>GPLGSETITVPTPIKQIFSDDAFAETIKDNLKKKSVTDAVTQNELNSIDQIIANNSDIKSVQGIQYLPNVTKLFLNGNKLTDIKPLANLKNLGWLFLDENKVKDLSSLKDLKKLKSLSLEHNGISDINGLVHLPQLESLYLGNNKITDITVLSRLTKLDTLSLEDNQISDIVPLAGLTKLQNLYLSKNHISDLRALAGLKNLDVLELFSQECLNKPINHQSNLVVPNTVKNTDGSLVTPEIISDDGDYEKPNVKWHLPEFTNEVSFIFYQPVTIGKAKARFHGRVTQPLKEVYTVSYDVDGT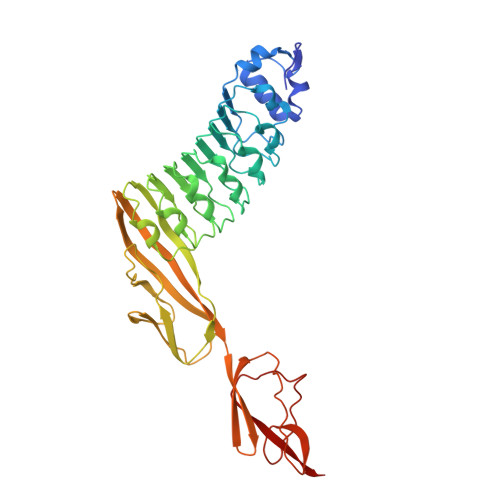VIKTKVEAGTRITAPKPPTKQGYVFKGWYTEKNGGHEWNFNTDYMSGNDFTLYAVFKAET[3x]>ASCTFTDAAAAIKGKASCTSIILNGIVVPAGTTLDMTGLKSGTTVTFQGKTTFGYKEWEGPLISFSGTNININGASGHSIDCQGSRWWDSKGSNGGKTKPKFF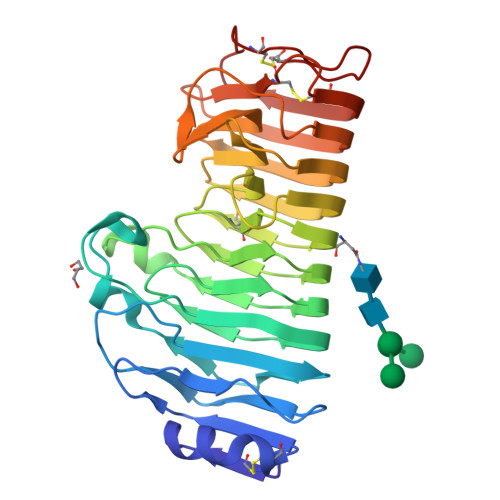YAHSLKSSNIKGLNVLNTPVQAFSINSATTLGVYDVIIDNSAGDSAGGHNTDAFDVGSSTGVYISGANVKNQDDCLAINSGTNITFTGGTCSGGHGLSIGSVGGRSDNTVKTVTISNSKIVNSDNGVRIKTVSGATGSVSGVTYSGITLSNIAKYGIVIEQDYENGSPTGTPTNGVPITGLTLSKITGSVASSGTNVYILCASGACSNWKWSGVSVTGGKKSTKCSNIPSGSGAAC[7x]> HHHHHHMTMTKQSSLSPGSRLYDYTTQDGAAWRVSALKEVSYDVVVQPRLLDPANPALADALSSGTTPARRLIVIDATVRSLYGEQLAAYLAGHDVEFHLCVIDAHESAKVMETVFEVVDAMDAFGVPRRHAPVL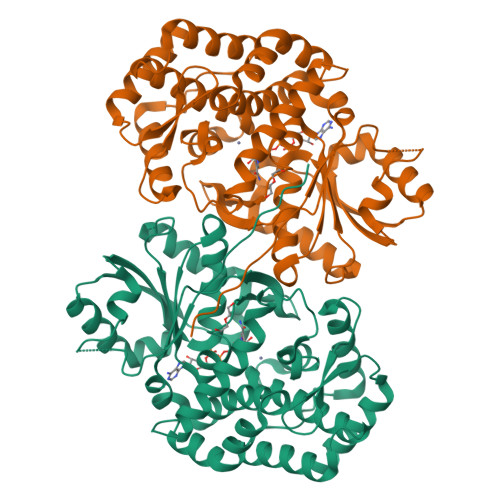AMGGGVLTDIVGLAASLYRRATPYVRIPTTLIGMIDAGIGAKTGVNFREHKNRLGTYHPSSLTLIDPGFLATLDARHLRNGLAEILKVALVKDAELFDLLEGHGASLVEQRMQPGEGGTGGAALTVLRRAVQGMLEELQPNLWEHQLRRLVDFGHSFSPSVEMAALPELLHGEAVCIDMALSSVLAHHRGLLTEAELGRVLDVMRLLHLPVLHPVCTPDLMRAALADTVKHRDGWQHMPLPRGIGDAVFVNDVTQREIEAALLTLAERDRVPRWRALHGAVDMGV>MGCWGRNRGRLLCMLALTFMFMVLEVVVSRVTSSLAMLSDSFHMLSDVLALVVALVAERFARRTHATQKNTFGWIRAEVMGALVNAIFLTGLCFAILLEAIERFIEPHEMQQPLVVLGVGVAGLLVNVLGLCLFHHHSGFSQDSGHGHSHGGHGHGHGLPKGPRVKSTRPGSSDINVAPGEQGPDQEETNTLVANTSNSNGLKLDPADPENPRSGDTVEVQVNGNLVREPDHMELEEDRAGQLNMRGVFLHVLGDALGSVIVVVNALVFYFSWKGCSEGDFCVNPCFPDPCKAFVEIINSTHASVYEAGPCWVLYLDPTLCVVMVCILLYTTYPLLKESALILLQTVPKQIDIRNLIKELRNVEGVEEVHELHVWQLAGSRIIATAHIKCEDPTSYMEVAKTIKDVFHNHGIHATTIQPEFASVGSKSSVVPCELACRTQCALKQCCGTLPQAPSGKDAEKTPAVSISCLELSNNLEKKPRRTKAENIPAVVIEIKNMPNKQPESSLSRLEEELRRRTEGGSSDLEVLFQ[2x]

ZnT/SLC30 transporters are major players in regulating zinc homeostasis, by harnessing the proton gradient to mobilize the divalent cationic zinc across membranes. ZIPs increase the cytosolic Zn2+ by either importing from the extracellular space or releasing the stored Zn2+ from subcellular compartments, whereas ZnTs remove Zn2+ out of the cytoplasm and maintain physiologically low free Zn2+. ZnT/YiiP mediated Zn2+ transport is mainly powered by proton gradient. Here we determined four high-resolution structures of the plasma-specific hZnT1 and the synaptic vesicle-specific hZnT3.

Local resolution analysis indicated density quality better than 2.5-Å for TMD Zn2+ sites (Fig. EV1B), which showed clear signs for Zn2+ ions present at both outward-facing TMD translocation funnels. Similar to the Zn2+-unbound OF/OF ZnT1 structure, three Zn2+-binding SCD sites were also identified in Zn2+-bound OF/OF ZnT1, without an additional TMD/CTD interface SIF site as seen in hZnT8 or bacterial YiiP structures when incubated with zinc (Fig. EV3A). The two Zn2+-bound protomers are well aligned. Notably, a short segment of TM2 extracellular half (residues 41–46) in both protomers adopts a stretched conformation (Figs. 3B and EV2C). As a result, zinc is chelated by three residues Asp47, His251 and Asp255, with His43 swinging away from the ion, which resembles the Zn2+-unbound apo state (trihedral-network). With Zn2+ supplementation at pH 7.5, the 2.65-Å resolution map reveals that both protomers retain the OF state with Zn2+ coordinated at TMD sites by trihedral ligand composition instead of tetrahedral network. When His43 was protonated, His43 sidechain became mobile and distant from Zn2+, and TM2 segment stretched (Movie EV2).> MEYTYDVVIIGSGGAGFSAGLEAIAAGRSAVIIEKMPIIGGNSLISGAEMNVAGSWVQKNMGITDSKELFISDTLKGGDFKGDPEMVKTMVDNAVGAAEWLRDYVKVEFYPDQLFQFGGHSVKRALIPKGHTGAEVISKFSIKADEVGLPIHTNTKAEKLIQDQTGRIVGVEAAHNGKTITYHAKRGVVIATGGFSSNMEMRKKYNPELDERYGSTGHAGGTGDGIVMAEKIHAAAKNMGYIQSYPICSPTSGAIAL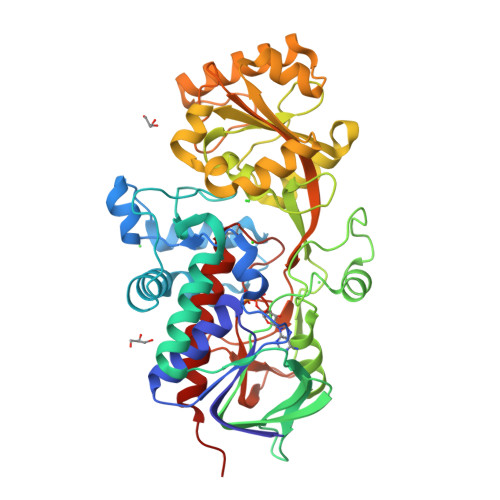IADSRFFGAVLINQKGERFVEELERRDVISHAILAQPGRYTYVLWNQDIENVAHTVEMHQGELKEFTKDGLMYKVDTLEEAAKVFNIPEDKLLSTIKDVNHYAATGKDEAFNHRSGLVDLSKGPYWILKATPSVHHTMGGLVVDTRTRVLDEQGKVIPGLFAAGEVTGLTHGTNRLGGNAYTDIIVYGRIAGQEAAKHHHHHH>MAREFSLEKTRNIGIIAHIDAGKTTTTERILYYTGRIHKIGETHEGASQMDWMEQEQDRGITITSAATTAAWEGHRVNIIDTPGHVDLTVEVERSLRVLDGAVTVLDAQSGVEPQTETVWRQATTYGVPRIVFVNKMDKLGANFEYSVSTLHDRLQANAAPIQLPIGAEDEFEAIIDLVEMKCFKYTNDLGTEIEEIEIPEDHLDRAEEARASLIEAVAETSDELMEKYLGDEEISVSELKEAIRQATTNVEFYPVLCGTAFKNKGVQLMLDAVIDYLPSPLDVKPIIGHRASNPEEEVIAKADDSAEFAALAFKVMTDPYVGKLTFFRVYSGTMTSGSYVKNSTKGKRERVGRLLQMHANSRQEIDTVYSGDIAAAVGLKDTGTGDTLCGEKNDIILESMEFPEPVIHLSVEPKSKADQDKMTQALVKLQEEDPTFHAHTDEETGQVIIGGMGELHLDILVDRMKKEFNVECNVGAPMVSYRETFKSSAQVQGKFSRQSGGRGQYGDVHIEFTPNETGAGFEFENAIVGGVVPREYIPSVEAGLKDAMENGVLAGYPLIDVKAKLYDGSYHDVDSSEMAFKIAASLALKEAAKKCDPVILEPMMKVTIEMPEEYMGDIMGDVTSRRGRVDGMEPRGNAQVVNAYVPLSEMF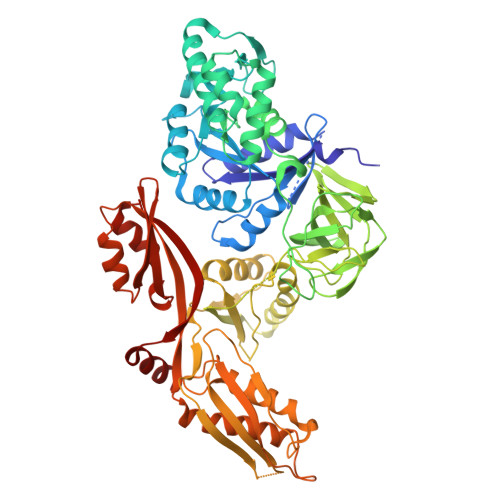GYATSLRSNTQGRGTYTMYFDHYAEVPKSIAEDIIKKNKGE[2x]>[4x]MGQNMEIDNFLKIERLAENDLPKFIQLIRLFEAVFEMKNFSIPDSEHLQKLLNQNNFYVFV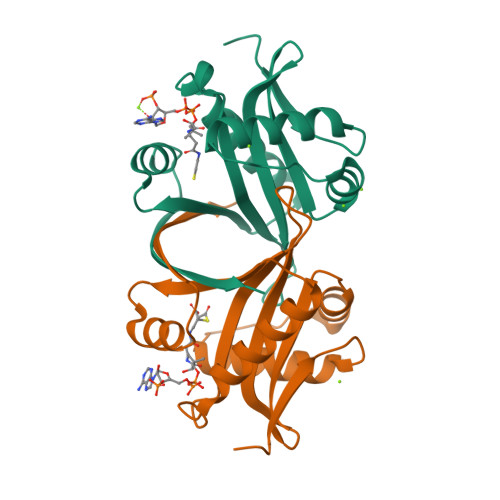ALLENKIVGGLTSYVLEQYYSEKPLAYIYDLAVDTNWQRQGIGKKLITATNQFYTEKGFEEVFVQADKVDDYALDFYRSTKPTAEEQVVHFYYTLK> MQNAESWFKKYWHLSVLVIAALISVKLRILNPWNSVFTWTVRLGGNDPWYYYRLIENTIHNFPHRIWFDPFTYYPYGSYTHFGPFLVYLGSIAGIIFSATSGESLRAVLAFIPAIGGVLAILPVYLLTREVFDKRAAVIAAFLIAIVPGQFLQRSILGFNDHHIWEAFWQVSALGTFLLAYNRWKGHDLSHNLTARQMAYPVIAGITIGLYVLSWGAGFIIAPIILAFMFFAFVLAGFVNADRKNLSLVAVVTFAVSALIYLPFAFNYPGFSTIFYSPFQLLVLLGSAVIAAAFYQIEKWNDVGFFERVGLGRKGMPLAVIVLTALIMGLFFVISPDFARNLLSVVRVVQPKGGALTIAEVYPFFFTHNGEFTLTNAVLHFGALFFFGMAGILYSAYRFLKRRSFPEMALLIWAIAMFIALWGQNRFAYYFAAVSAVYSALALSVVFDKLHLYRALENAIGARNKLSYFRVAFALLIALAAIYPTYILADAQSSYAGGPNKQWYDALTWMRENTPDGEKYDEYYLQLYPTPQSNKEPFSYPFETYGVISWWDYGHWIEAVAHRM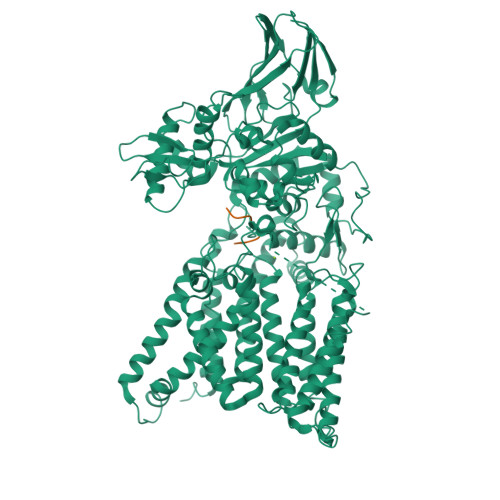PIANPFQAGIGNKYNNVPGASSFFTAENESYAEFVAEKLNVKYVVSDIEMETCKYYAMAVWAEGDLPLAEKYYGGYFYYSPTGTFGYANSQWDIPLNSIIIPLRIPSELYYSTMEAKLHLFDGSGLSHYRMIYESDYPAEWKSYSSQVNLNNESQVLQTALYEAVMRARYGVSPTMGTQEVLYKYAYTQLYEKKMGIPVKIAPSGYVKIFERVKGAVVTGKVSANVTEVSVNATIKTNQNRTFEYWQTVEVKNGTYTVVLPYSHNSDYPVKPITPYHIKAGNVVKEITIYESQVQNGEIIQLDLELALVPR;> RYNVTAC> MRLESVAKFHSPKSPMMSDSPRATASDSLSGTDVMAAMGMAQSQAGFGMAAFCGKHELSQNDKQKAINYLMQFAHKVSGKYRGVAKLEG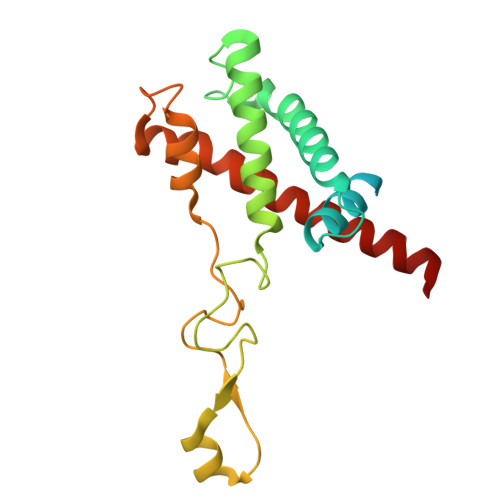NTKAKVLQVLATFAYADYCRSAATPGARCRDCHGTGRAVDIAKTELWGRVVEKECGRCKGVGYSRMPASAAYRAVTMLIPNLTQPTWSRTVKPLYDALVVQCHKEESIADNILNAVTR> EDRPIKFSTEGATSQSYKQFIEALRERLRGGLIHDIPVLPDPTTLQERNRYITVELSNSDTESIEVGIDVTNAYVVAYRAGTQSYFLRDAPSSASDYLFTGTDQHSLPFYGTYGDLERWAHQS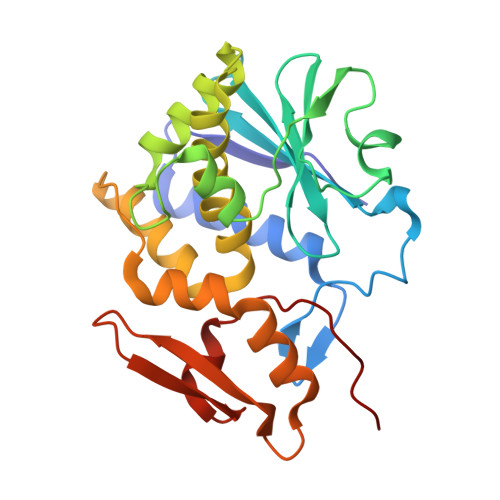RQQIPLGLQALTHGISFFRSGGNDNEEKARTLIVIIQMVAEAARFRYISNRVRVSIQTGTAFQPDAAMISLENNWDNLSRGVQESVQDTFPNQVTLTNIRNEPVIVDSLSHPTVAVLALMLFVCNPPN1-{2-[3-(2-Chloro-4,5-difluoro-benzoyl)-ureido]-4-fluoro-phenyl}-piperidine-4-carboxylic 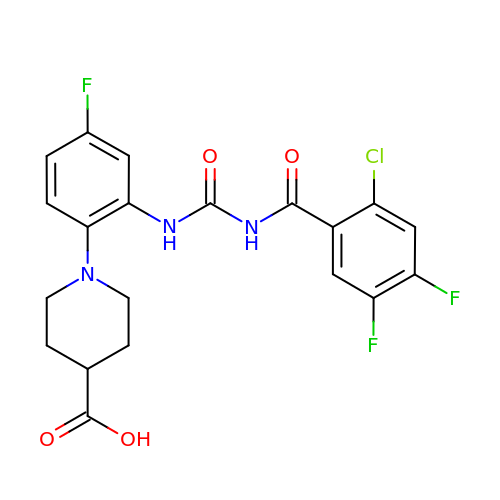acid | C20 H17 Cl F3 N3 O4 | KAJJGOCSAXKXBD-UHFFFAOYSA-N>MGSSHHHHHHSSGRENLYFQGHDGEEDEIVQREDGSWLVDGMVSLDRFREFFELEAPLPGEAGGNIHTLAGVMLYQLGRV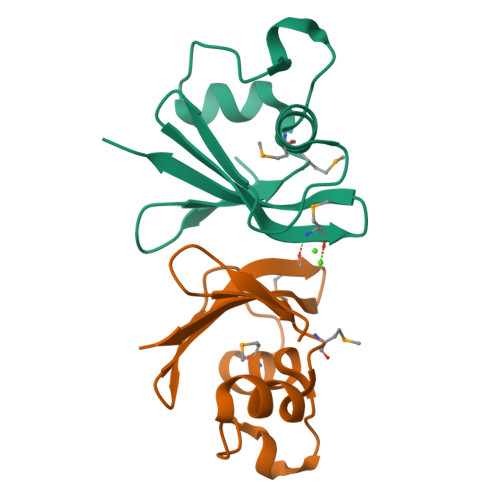PSVTDRFEWNGFSFEVVDMDRTRVDKILVQRHH[6x]2-[[2,6-bis(chloranyl)-4-pyridin-4-yl-phenyl]amino]benzoic acid | C18 H12 Cl2 N2 O2 | 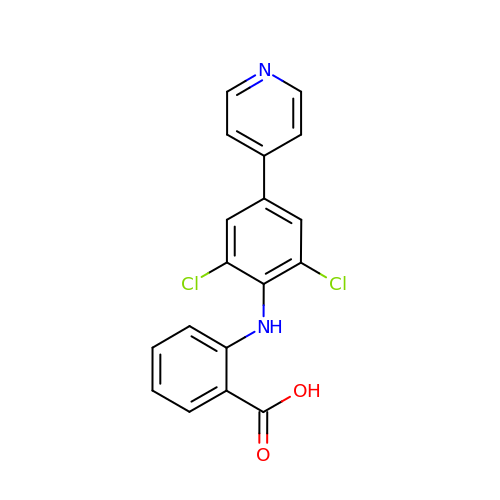GSNZPZDSMBVGPU-UHFFFAOYSA-N>MKGKMAIVISTLNNPWFVVLAETAKQRAEQLGYEATIFDSQNDTAKESAHFDAIIAAG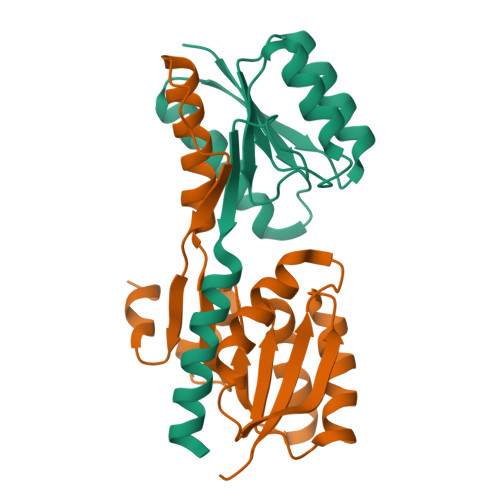YDAIIFNPTDADGSIANVKRAKEAGIPVFCVDRGINARGLAVAQIYSDNYYGGVLMGEYFVKFLKEKKLEHHHHHH[2x];>[2x]MGEYFVKFLKEKYPDAKEIPYAELLGILSAQPTWDRSNGFHSVVDQYPEFKMVAQQSAEFDRDTAYKVTEQILQAHPEIKAIWCGNDAMALGAMKACEAAGRTDIYIFGFDGAEDVINAIKEGKQIVATIMQFPKLMARLAVEWADQYLRGERSFPEIVPVTVELVTRENIDKYTAYGRKLEHHHHHH>MTLLSPGIELKETTVQSTVVNNSTGTAALAGKFQWGPAFQIK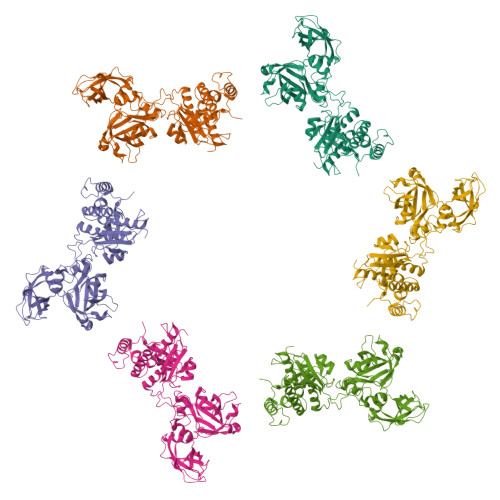QVTNEVDLVNTFGQPTAETADYFMSAMNFLQYGNDLRVVRAVDRDTAKNSSPIAGNIEYTISTPGSNYAVGDKITVKYVSDDIETEGKITEVDADGKIKKINIPTAKIIAKAKEVGEYPTLGSNWTAEISSSSSGLAAVITLGKIITDSGILLAEIENAEAAMTAVDFQANLKKYGIPGVVALYPGELGDKIEIEIVSKADYAKGASALLPIYPGGGTRASTAKAVFGYGPQTDSQYAIIVRRNDAIVQSVVLSTKRGGKDIYDSNIYIDDFFAKGGSEYIFATAQNWPEGFSGILTLSGGLSSNAEVTAGDLMEAWDFFADRESVDVQLFIAGSCAGESLETASTVQKHVVSIGDVRQDCLVLCSPPRETVVGIPVTRAVDNLVNWRTAAGSYTDNNFNISSTYAAIDGNYKYQYDKYNDVNRWVPLAADIAGLCARTDNVSQTWMSPAGYNRGQILNVIKLAIETP[6x]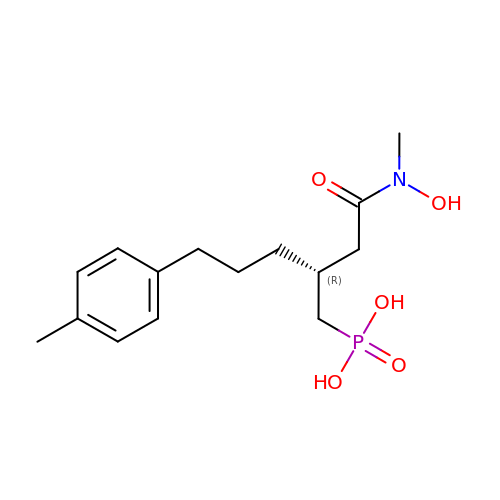[(2R)-2-{2-[hydroxy(methyl)amino]-2-oxoethyl}-5-(4-methylphenyl)pentyl]phosphonic acid | C15 H24 N O5 P | PCPXBXKPZNRAMA-CQSZACIVSA-N> MFKIVYPNAKDFFSFINSITNVTDSIILNFTEDGIFSRHLTEDKVLMAIMRIPKDVLSEYSIDSPTSVKLDVSSVKKILSKASSKKATIELTETDSGLKIIIRDEKSGAKSTIYIKAE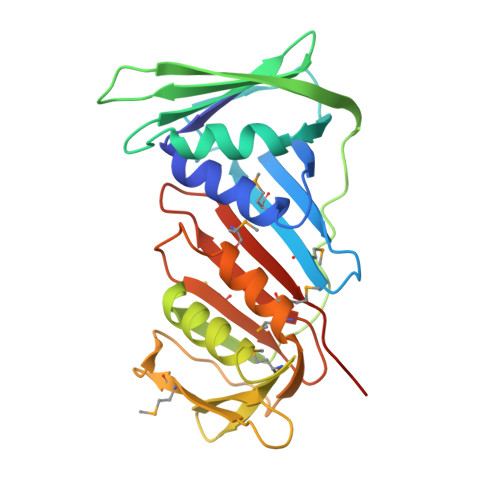KGQVEQLTEPKVNLAVNFTTDESVLNVIAADVTLVGEEMRISTEEDKIKIEAGEEGKRYVAFLMKDKPLKELSIDTSASSSYSAEMFKDAVKGLRGFSAPTMVSFGENLPMKIDVEAVSGGHMIFWIAPRLLEHHHHHH> GDQVEQSPSALSLHEGTDSALRCNF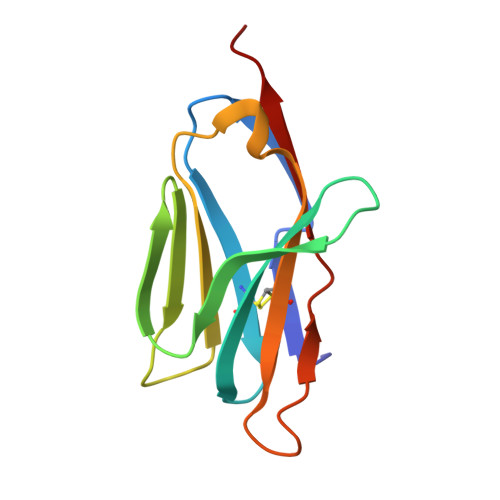TTTMRSVQWFRQNSRGSLISLFYLASGTKENGRLKSAFDSKERRYSTLHIRDAQLEDSGTYFCAAEASSGSWQLIFGSGTQLTVMPVT(3S)-3-(2H-1,3-benzodioxol-5-yl)-1-[(3R,5S)-3,5-dimethylpiperidin-1-yl]-3-(2-hydroxy-4,6-dimethoxyphenyl)propan-1-one | C25 H31 N O6 | 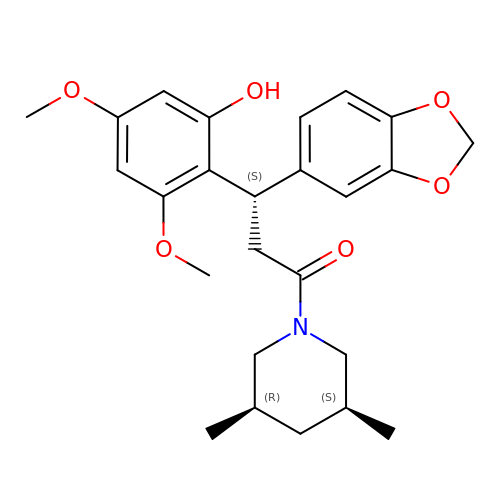YEKVAIMYYCZDLI-FCEWJHQRSA-N(2R)-3-hydroxypropane-1,2-diyl dihexanoate | C15 H28 O5 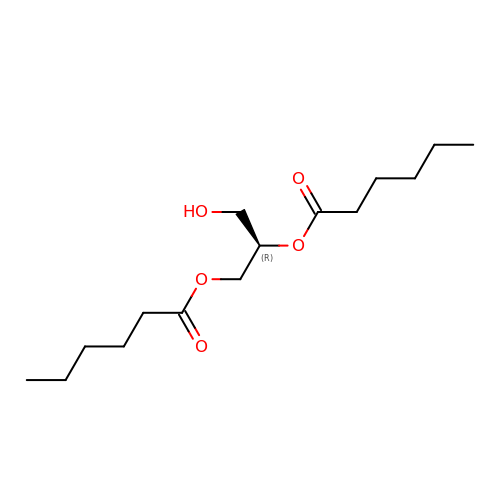| DRUFTGMQJWWIOL-CYBMUJFWSA-N>MEKILIFGHQNPDTDTICSAIAYADLKNKLGFNAEPVRLGQVNGETQYALDYFKQESPRLVETAANEVNGVILVDHNERQQSIKDIEEVQVLEVIDHHRIANFETAEPLYYRAEPVGCTATILNKMYKENNVKIEKEIAGLMLSAIISDSLLFKSPTCTDQDVAAAKELAEIAGVDAEEYGLNMLKAGADLSKKTVEELISLDAKEFTLGSKKVEIAQVNTVDIEDVKKRQAELEAVISKVVAEKNLDLFLLVITDILENDSLALAIGNEAAKVEKAFNVTLENNTALLKGVVS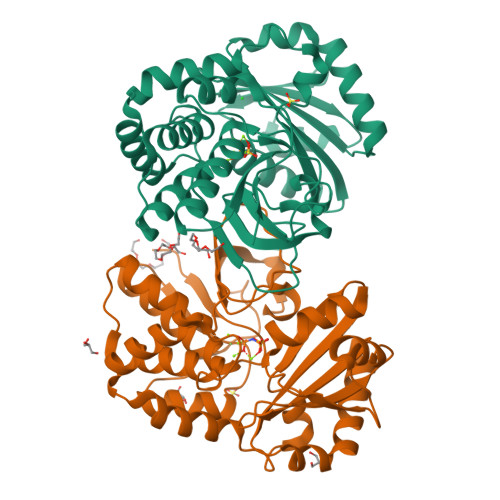RKKQVVPVLTDAMAE[2x]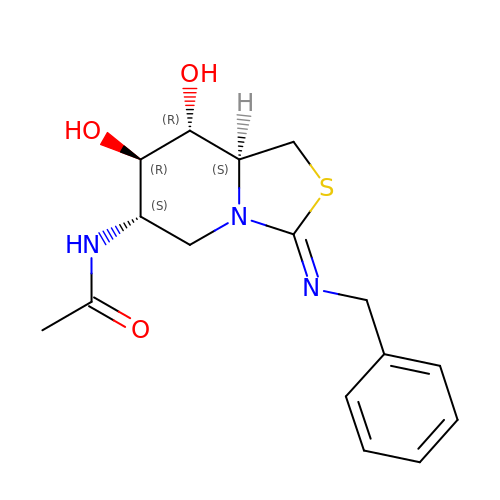~{N}-[(3~{Z},6~{S},7~{R},8~{R},8~{a}~{S})-7,8-bis(oxidanyl)-3-(phenylmethyl)imino-1,5,6,7,8,8~{a}-hexahydro-[1,3]thiazolo[3,4-a]pyridin-6-yl]ethanamide | C16 H21 N3 O3 S | DWUFYAAHHCWFAW-OZFNUUMKSA-N>CUCCUCCGCGCG[2x];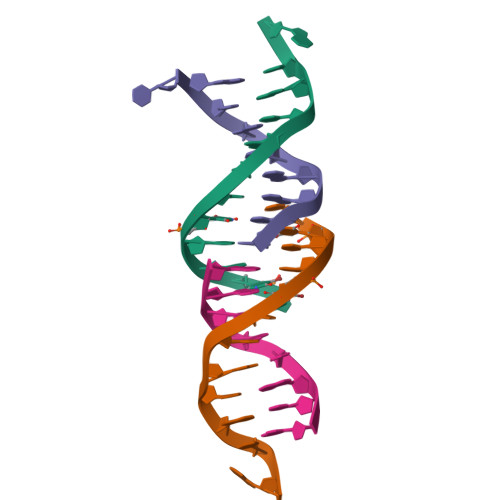>[2x]CGCGCGGAG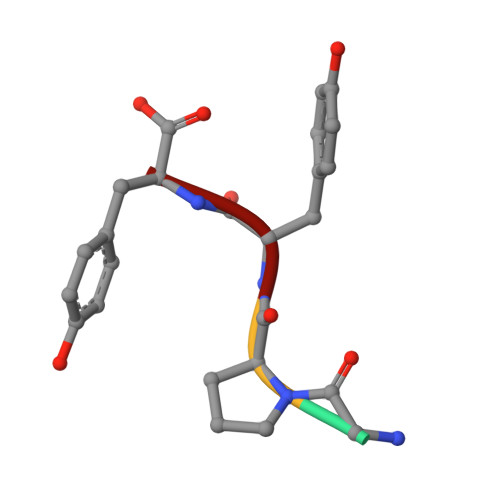> GPYY> MGTATDNARQVTIIGAGLAGTLVARLLARNGWQVNLFERRPDPRIETGARGRSINLALAERGAHALRLAGLEREVLAEAVMMRGRMVHVPGTPPNLQPYGRDDSEVIWSINRDRLNRILLDGAEAAGASIHFNLGLDSVDFARQRLTLSNVSGERLEKRFHLLIGADGCNSAVRQAMASVVDLGEHLETQPHGYKELQITPEASAQFNLEPNALHIWPHGDYMCIALPNLDRSFTVTLFLHHQSPAAQPASPCFAQLVDGHAARRFFQRQFPDLSPMLDSLEQDFEHHPTGKLATLRLTTWHVGGQAVLLGDAAHPMVPFHGQGMNCALEDAVALAEHLQSAADNASALAAFTAQRQPDALAIQAMALENYVEMSSKVASPTYLLERELGQIMAQRQPTRFIPRYSMVTFSRLPYAQAMARGQIQEQLLKFAVANHSDLTSINLDAVEHEVTRCLPPLSHLCAAALEH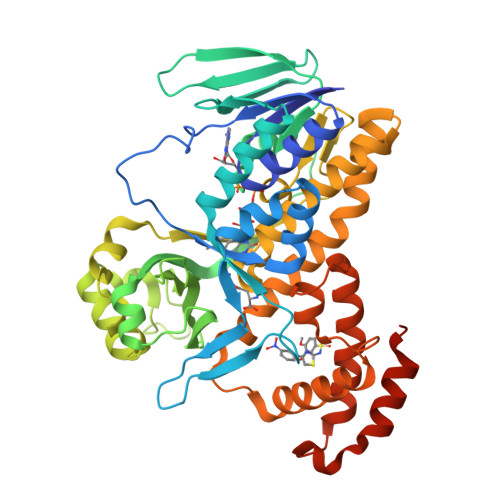HHHHH Using several techniques, we show that electron paramagnetic resonance (EPR) spectroscopy of oligonucleotides spin-labelled with triazole-appended nitroxides at the 2′ position offers a robust and minimally perturbing tool for obtaining such measurements. Here we address this challenge through a synergistic combination of EPR spectroscopy, X-ray crystallography, NMR spectroscopy and MD simulations, which accurately identify spin label location on a DNA duplex. As well as affording the first X-ray crystallographic structures of B-form spin-labelled DNA duplexes, the combination of these four techniques demonstrates the minimally perturbing nature of deoxynucleic acid 2′-spin-labelling. Using experimental and computational methods to support EPR spectroscopic observations, we demonstrate that spin-labelling of DNA via 2′-triazole-linked nitroxides is minimally perturbing and affords DEER data with narrow (sub-nanometre) distance distributions due to well-defined minor groove nitroxide conformations.

Nevertheless, the X-ray structures of both the double 6-Me-labelled duplex 6 and single 5-Me-labelled duplex 7 revealed that the triazole-nitroxide occupies the minor groove of the duplexes. The electron density of all residues is well-defined, but only a small amount of density is seen for the 5-Me spin label, corresponding to the triazole. The lack of density is likely due to dynamic disorder associated with the methylene linker. Although the pyrroline ring is not resolved, the triazole is again observed to adopt a conformation with its N3 atom situated under the deoxyribose ring. By contrast, superposition of the X-ray structures of duplexes 7 and 8 shows that their overall geometry is highly conserved. Although duplexes 6 and 7 exhibit overall B-form geometry, some local structural parameters varied at the modified uridines. Most notably, the puckering and glycosyl torsion angles of these residues are A-form-like: the pseudorotation phase angles P of the 6U sugars are 49° and 36° (C4′-exo and C3′-endo), and 45° for the 5U sugar (C4′-exo), whilst the glycosyl torsion angles are –141° and –146° for the 6Us, and –146° for 5U. The similarity of the spin-labelled uridine phase angles, despite differences in their crystalline environments, suggests that the observed pucker represents a major conformer rather than a crystal-packing effect. Importantly, the perturbations in duplexes 6 and 7 are localized at the modified nucleotides and do not propagate along the duplex, which would have significant implications for the EPR distance distributions.

> CGCAAAAAAGCG;> CGCTTTTTXGCG6-[(3-hydroxybenzyl)amino]pyridine-3-carboxamide | C13 H13 N3 O2 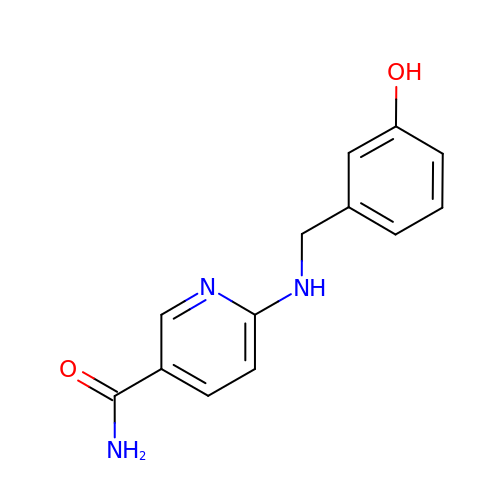| WNJXCRUMIMMAQO-UHFFFAOYSA-N> SNAMSSKIPAVTYPKNESTPPSEELELDKWKTTMKSSVQEECVSTISSSKDED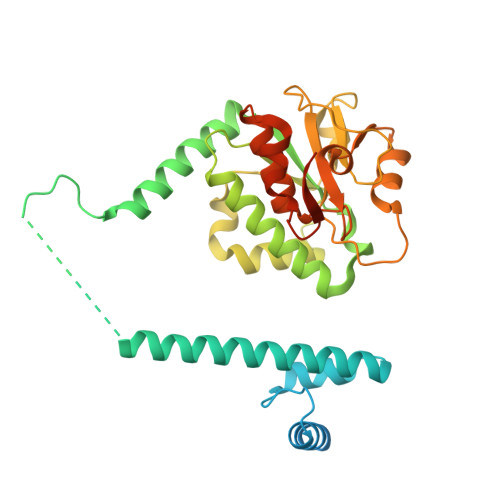PLAATREFIEMWRLLGREVPEHITEEELKTLMECVSNTAKKKYLKYLYTKEKVKKARQIKKEMKAAAREEAKNIKLLETTEEDKQKNFLFLRLWDRNMDIAMGWKGAQAMQFGQPLVFDMAYENYMKRKELQNTVSQLLESEGWNRRNVDPFHIYFCNLKIDGALHRELVKRYQEKWDKLLLTSTEKSHVDLFPKDSIIYLTADSPNVMTTFRHDKVYVIGSFVDKSMQPGTSLAKAKRLNLATECLPLDKYLQWEIGNKNLTLDQMIRILLCLKNNGNWQEALQFVPKRKHTGFLEISQHSQEFINRLKKAKT>[6x]MRFI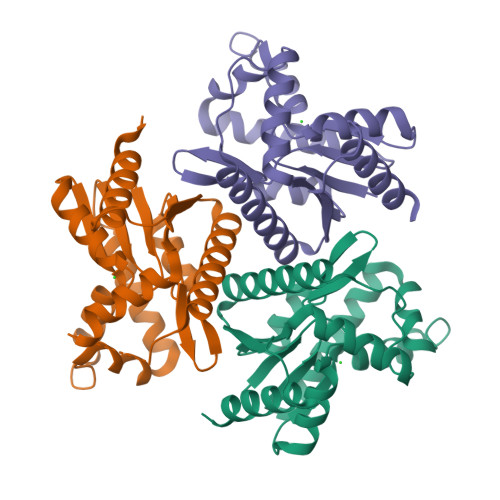LTGVPGAGKTTVCNKLAEKMSNLSVVNYGDVIFEEAKKLYPSIIQVREDTRKLPRADYRNIQIEAAKKISLITDNLIVDTHMSLKTPYGFYPGLIPETINIIQPDGIILLEFNPRDVIARREKDRLAGKRVTRDMESETDILLHQQVNRMFAVSYSAINQCYVKIIDLTWPQEYEFQHTEYAVNKIIEMLNFKI> VPEAPTPMWPDDLQNHTFLHTVYCQDGSPSVGLSEAYDEDQLFFFDFSQNTRVPRLPEFADWAQEQGDAILFDKEFCEWMIQQIPKLDGKIPVSRGFPIAEVFTLKPLEFGKPNTLVCFVSNLFPPMLTVNWH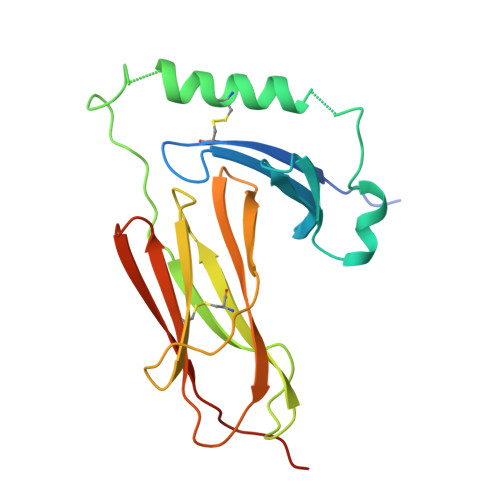DHSVPVEGFGPTFVSAVDGLSFQAFSYLNFTPEPSDIFSCIVTHEPDRYTAIAYWVPRNALPSDLLEN(5S)-5-[(1R)-1-(4-chloranyl-1H-indol-3-yl)ethyl]-2-(methylamino)-1,3-oxazol-4-one | C14 H14 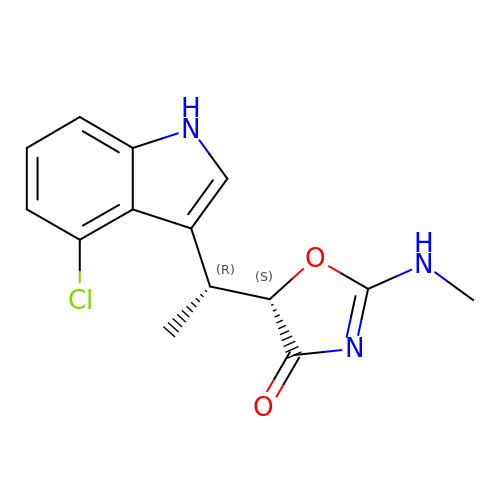Cl N3 O2 | YMXVJMTTWGZCKW-KRTXAFLBSA-N(+)-menthone | C10 H18 O | 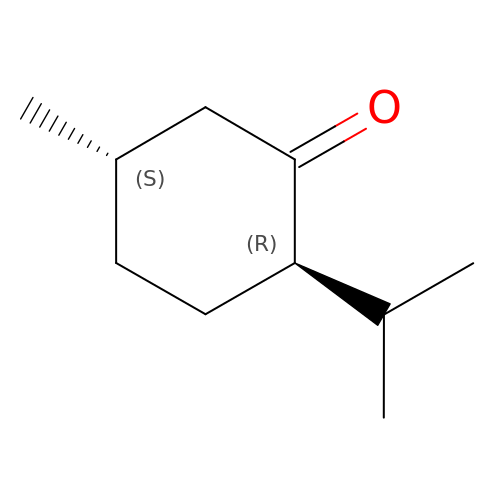NFLGAXVYCFJBMK-DTWKUNHWSA-N>GSHMNGNNTSETQGDRTEQAETVQADLFSADSAYTFVQRQVNFGPRIPGTAPH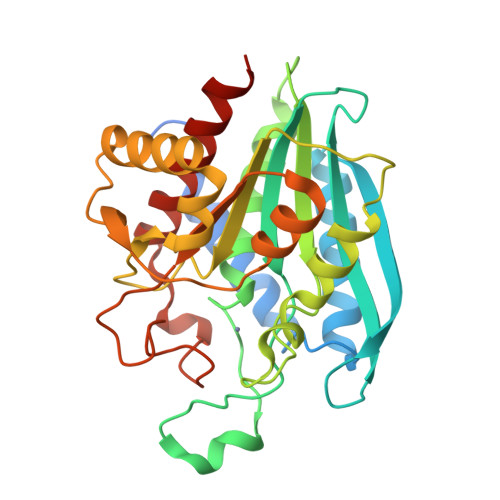RACGDWLVATLRSFGAAVQEQTAEIKAHDGTMLPMRNIIASYRPEATGRMLLMAHWDTRPVCDQDANPAMHTETFDGADDGGSGVGVLLEIARYLGQQKDLGMGIDIVFFDTEDYGSYGDDESWCLGSQYWSRNPHVAGYKAEAGILLDMVGAKGATFYWEYFSKSYAPGLISAVWQTAAALGYGNYFIQADGGALTDDHVPVIKNLGIPCIDIINYSSKNEHGFGDHWHTQRDNMQIIDKNVLDAVGETVIRYLDEQVKAASH[2x]> IRLTNQLKSLKGLQSKLKDVVEYLDKVINK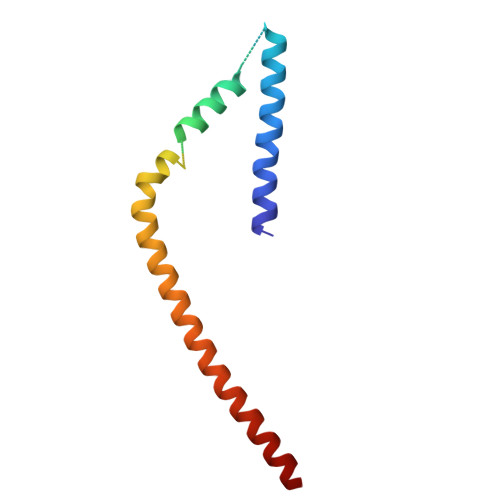ELPINHTILGKLQDVFNLLPNLGTPDDDEIDVENHDRINISNNLQKALTVKTNDELMVIYISNLVRSIIAFDDLIENKIQNKKIQEQRVKD> DGARRKRVLHDACVCGWMIEFLQAHYLVEDDIMDNSVTRRGKPCWYRHPDVTVQCAINDGLLLKSWTHMMAMHFFADRPFLQDLLCRFNRVDYTTAVGQLYDVTSMFDSNKLDPDVSQPTTTDFAEFTLSNYKRIVKYKTAYYTYLLPLVMGLIVSEALPTVDMGVTEELAMLMGEYFQVQDDVMDCFTPPERLGKVGTDIQDAKCSWLAVTFLAKASSAQVAEFKANYGSGDSEKVATVRRLYEEADLQGDYV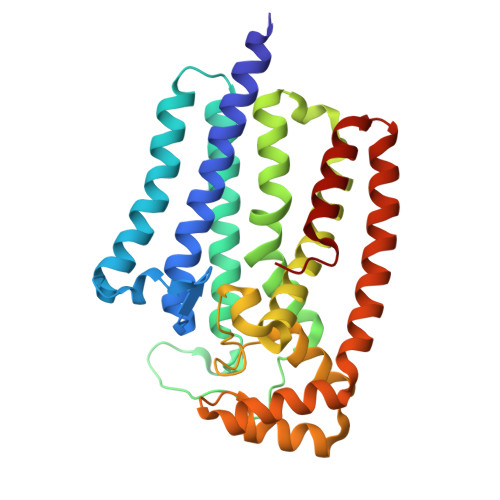AYEAAVAEQVKELIEKLRLCSPGFAASVETLWGKTYKRQK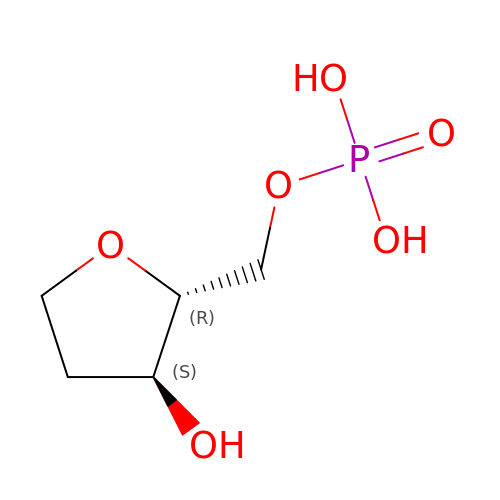1',2'-DIDEOXYRIBOFURANOSE-5'-PHOSPHATE | C5 H11 O6 P | BVOBPNSQIRMLCA-CRCLSJGQSA-N> GPLGSQMT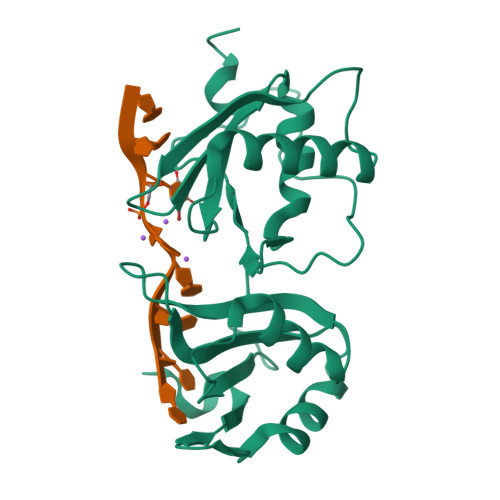RQARRLYVGNIPFGITEEAMMDFFNAQMRLGGLTQAPGNPVLAVQINQDKNFAFLEFRSVDETTQAMAFDGIIFQGQSLKIRRPHDYQPLPGMSENPSVYVPGVVSTVVPDSAHKLFIGGLPNYLNDDQVKELLTSFGPLKAFNLVKDSATGLSKGYAFCEYVDINVTDQAIAGLNGMQLGDKKLLVQRASVGAKN>MESKRNKPGKATGKGKPVGDKWLDDAGKDSGAPIPDRIADKLRDKEFKSFDDFRKAVWEEVSKDPELSK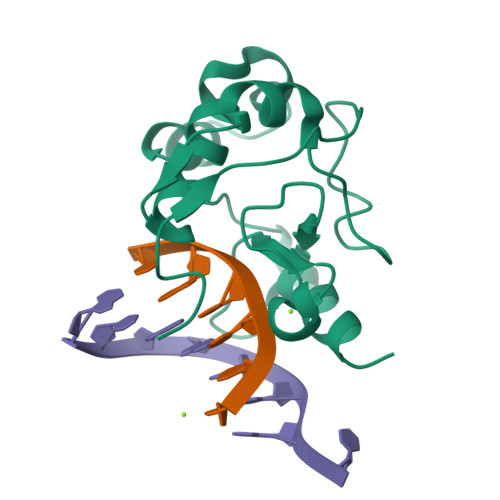NLNPSNKSSVSKGYSPFTPKNQQVGGRKVYELHADKPISQGGEVYDMDNIRVTTPKRHIDIHRGK[4x]>WTNTSGSCRGRCFERTFSNCRCDAACVSLGNCCLDFQETCVEPTHIWTCNKFRCGEKRLSRFVCSCADDCKTHNDCCINYSSVCQDKKSWVEETCESIDTPECPAEFESPPTLLFSLDGFRAEYLHTWGGLLPVISKLKNCGTYTKNMRPMYPTKTFPNHYSIVTGLYPESHGIIDNKMYDPKMNASFSLKSKEKFNPLWYKGQPIWVTANHQEVKSGTYFWPGSDVEIDGILPDIYKVYNGSVPFEERILAVLEWLQLPSHERPHFYTLYLEEPDSSGHSHGPVSSEVIKALQKVDRLVGMLMDGLKDLGLDKCLNLILISDHGMEQGSCKKYVYLNKYLGDVNNVKVVYGPAARLRPTDVPETYYSFNYEALAKNLSCREPNQHFRPYLKPFLPKRLHFAKSDRIEPLTFYLDPQWQLALNPSERKYCGSGFHGSDNLFSNMQALFIGYGPAFKHGAEVDSFENIEVYNLMCDLLGLIPAPNNGSHGSLNHLLKKPIYNPSHPKEEGFLSQCPIKSTSNDLGCTCDPWIVPIKDFEKQLNLTTEDDDIYHMTVPYGRPRILLKQHRVCLLQQQQFLTGYSLDLLMPLWASYTFLSNDQFSRDDFSNCLYQDLRIPLSPVHKCSYYKSNSKLSYGFLTPPRLNRVSNHIYSEA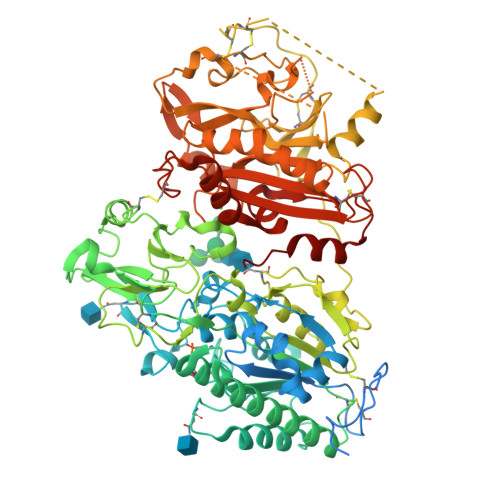LLTSNIVPMYQSFQVIWHYLHDTLLQRYAHERNGINVVSGPVFDFDYDGRYDSLEILKQNSRVIRSQEILIPTHFFIVLTSCKQLSETPLECSALESSAYILPHRPDNIESCTHGKRESSWVEELLTLHRARVTDVELITGLSFYQDRQESVSELLRLKTHLPIFSQED[2x]> SVVANYDQMMRVPIQRRAKVMSIRGERSYNTPLGKVAMKNGLSDKDMKDVSADLVISTVTAPRTDPAGTGAENSNMTLKILNNTGVDLLINDITVRPTVIAGNIKGNTMSNTYFSSKDIKSSSSKITLIDVCSKFEDG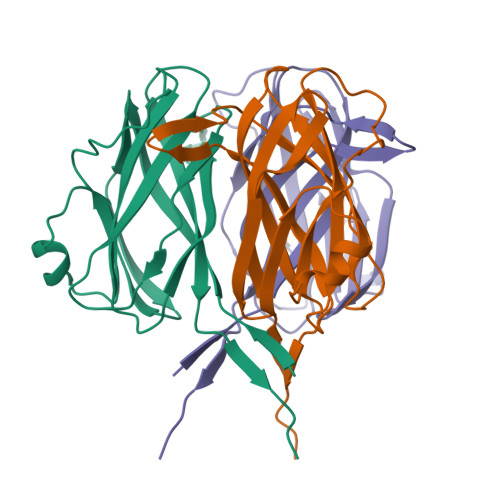AAFEATMNIGFTSKNVIDIKDEI>[3x]MFESMKPHLAELRQRLAISVLAVFVGFIIAFTFHNAILGWITKPLNNALIQVGKIVEKREMGTWKISGNEHNATLAPSKSPALLSDHAQSAEKLHRTLAEASQATQNPKLQKLLSQAASAAEELARNSRILRKALVKEENLTRQ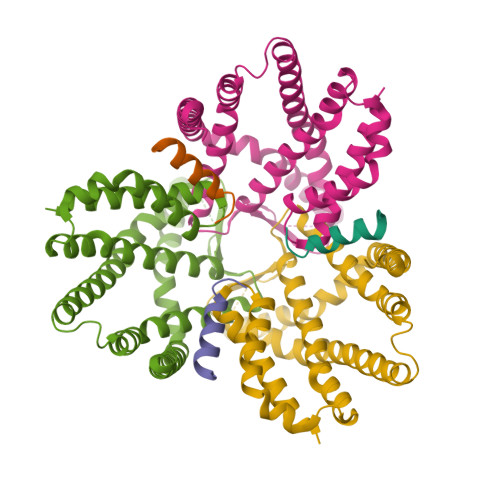AVNQNLREKSFNGMITTHQVGGAFFVALKVSFFAGILMAMPVILWQLWLFIAPGLYDNEKKMVLPFVVGGSVMFLIGVLFAYYVVTPFGFQFLITFGSFLYTPLINIEDYVGFFTKILIGFGIAFELPVVAYFLALLGLITDKTLKDYFKYAIVIIFLLAAFLTPPDVLTQLLMAAPLILLYGLSILIVHYVNPYKPEEKEDDEEEEEDEFEKAEREFEALEKGSESHESGSENLYFQ;>MGMPSGWELLLVVGVIVLLFGGKKIPELAKGLGKGIKDFKQAVKEDEEASAPAKEIENKEASASGTQSEASEVKESQKAWSHPQFEK[3x]>[2x]MENTENSVDSKSIKNLEPKIIHGSESMDSGISLDNSYKMDYPEMGLCIIINNKNFHKSTGATSRSGTDVDAANLRETFRNLKYEVRNKNDLTREEIVELMRDVSKEDHSKRSSFVCVLLSHGEEGIIFGTNGPV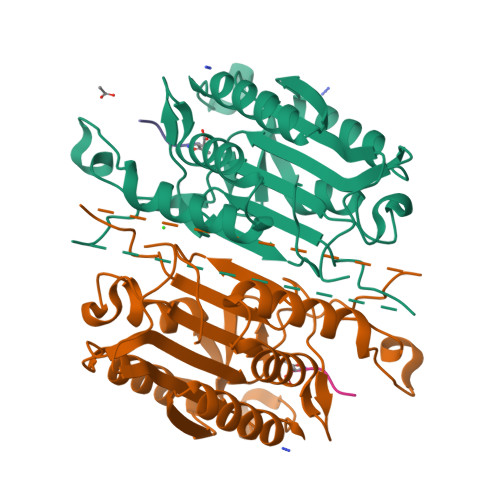DLKKITNFFRGDRCRSLTGKPKLFIIQACRGTELDCGIETDSGVDDDMACHKIPVEADFLYAYSTAPGYYSWRNSKDGSWFIQSLCAMLKQYADKLEFMHILTRVNRKVATEFESFSFDATFHAKKQIPCIVSMLTKELYFYH>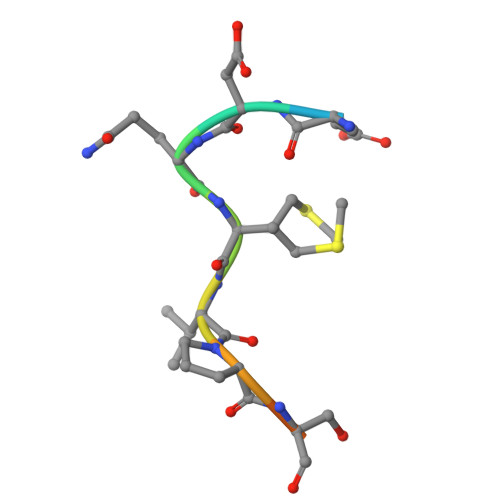 XEDQMVPSITY>[4x]MRGSHHHHHHYVAALFFLIPLVALGFAAANFAAVVRKPEGTERMKEISSYIRSGADSFLAHETKAIFKVAIVIAILLMIFTTWQTGVAFLLGAVMSASAGIVGMKMATRANVRVAEAARTTKKIGPALKVAYQGGSVMGLSVGGFALLGLVLVYLIFGKWMGQVDNLNIYTNWLGINFVPFAMTVSGYALGCSIIAMFDRVGGGVYTKAADMAADLVGKTELNLPEDDPRNPATIADNVGDNVGDVAGLGADLLESFVGAIVSSIILASYMFPIYVQKIGENLVHQVPKETIQALISYPIFFALVGLGCSMLGILYVIVKKPSDNPQRELNISLWTSALLTVVLTAFLTYFYLKDLQGLDVLGFRFGAISPWFSAIIGIFSGILIGFWAEYYTSYRYKPTQFLGKSSIEGTGMVISNGLSLGMKSVFPPTLTL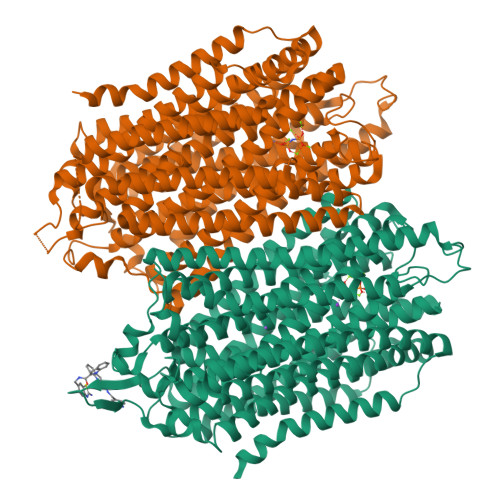VLGILFADYFAGLYGVAIAALGMLSFVATSVSVDSYGPIADNAGGISEMCELDPEVRKITDHLDAVGNTTAAIGKGFAIGSAIFAALSLFASYMFSQISPSDIGKPPSLVLLLNMLDARVIAGALLGAAITYYFSGYLISAVTKAAMKMVDEIRRQAREIPGLLEGKAKPDYNRCIEITSDNALKQMGYPAFIAILTPLVTGFLLGAEFVGGVLIGTVLSGAMLAILTANSGGAWDNAKKYLEAGNLEGYGKGSEPHKALVIGDTVGDPLKDTVGPSLDILIKIMSVVSVIAVSIFKHVHLF> SGRPSFAGKEYSLEPIDERTPILFQWFEARPERYEKGEVPILNTKEHPYLSNIINAAKIENERIIGVLVDGNFTYEQKKEFLNLENEHQNIAIIYRADVDFSMYDKKLSDIYLENIHKQESYPASERDNYLLGLLREELKNIPEGKDSLIESYAEKREHTWFDFFRNLAILKAGSLFTETGKTGCHNI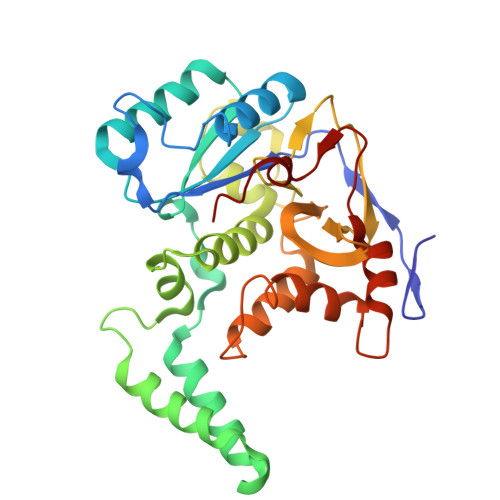SPCSGCIYLDADMIITDKLGVLYAPDGIAVHVDCNDEIKSLENGAIVVNRSNHPALLAGLDIMKSKVDAHPYYDGLGKGIKRHFNYSSLHNYNAFCDFIEFKHENIIPNTSMYTSSSW> MRFETLLKRAAQVGALVLLPLAAHAQEASAVDPARV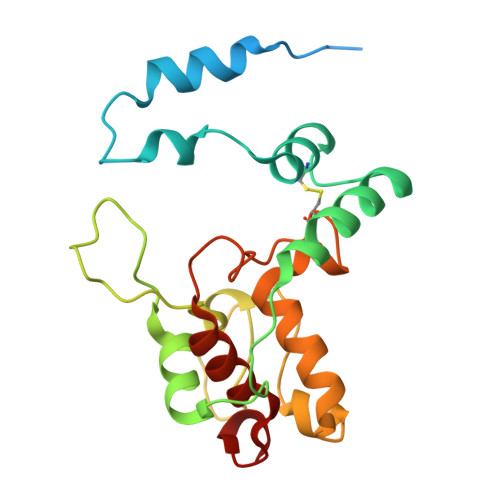DAVVKTSFTKLPEGWESRLQQDETQRICSVTRNNPSPEQAAAIMKAEEVRIKFPAGPVLGSWKDGAKVAQNGRGGQFSDPPGTVSGGNCYACHQLDPKEVSYGTLGPSLVGYGRERNFSAEDAKIAFAKVYDAQASLACSSMPRFGVNGVLTEQQIKDVVAYLFDPESPVNK2-(3-CARBOXYPROPIONYL)-6-HYDROXY-CYCLOHEXA-2,4-DIENE CARBOXYLIC ACID | C11 H12 O6 | 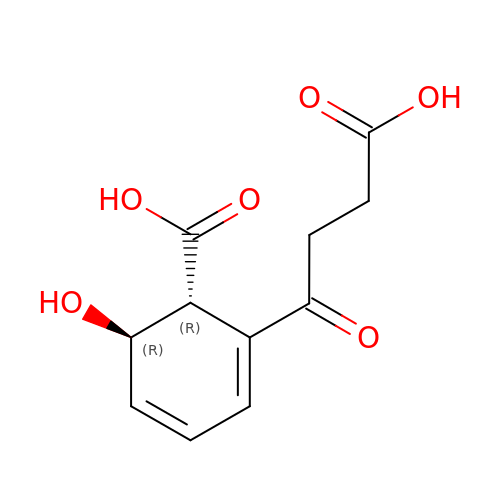QJYRAJSESKVEAE-PSASIEDQSA-N>YDNREIVMKYIHYKLSQRGYEWDAGADSEVVHKTLREAGDDFSRRYRRDFAEMSSGLHLTPFTARGRFATVVEELFRDGVNWGRIVAFFEFGGVMCVESVNREMSP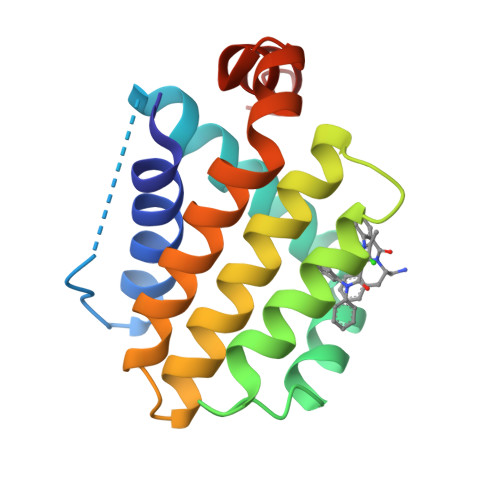LVDNIALWMTEYLNRHLHTWIQDNGGWDAFVELYGPSM[2x]>MAHYPPSKDQLNELIQEVNQWAITNGLSMYPPKFEENPSNASVSPVTIYPTPIPRKCFDEAVQIQPVFNELYARITQDMAQPDSYLHKTTEALALSDSEFTGKLWSLYLATLKSAQYKKQNFRLGIFRSDYLIDKKKGTEQIKQVEFNTVSVSFAGLSEKVDRLHSYLNRANKYDPKGPIYNDQNMVISDSGYLLSKALAKAVESYKSQQSSSTTSDPIVAFIVQRNERNVFDQKVLELNLLEKFGTKSVRLTFDDVNDKLFIDDKTGKLFIRDTEQEIAVVYYRT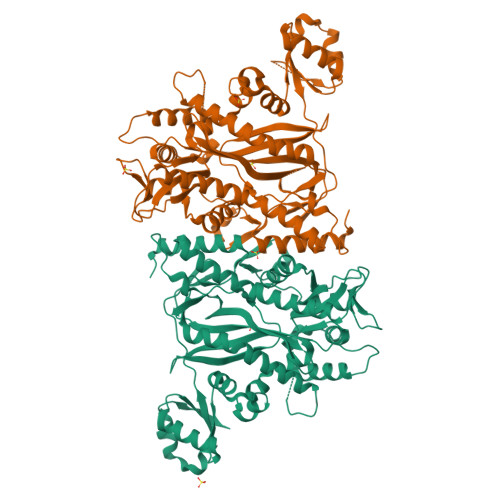GYTTTDYTSEKDWEARLFLEKSFAIKAPDLLTQLSGSKKIQQLLTDEGVLGKYISDAEKKSSLLKTFVKIYPLDDTKLGREGKRLALSEPSKYVLKPQREGGGNNVYKENIPNFLKGIEERHWDAYILMELIEPELNENNIILRDNKSYNEPIISELGIYGCVLFNDEQVLSNEFSGSLLRSKFNTSNEGGVAAGFGCLDSIILY[2x]The HAdV-D36 fiber knob domain (FK), which mediates the primary attachment of many HAdVs to host cells, has a significantly elongated DG loop that alters known binding interfaces for established adenovirus receptors such as the coxsackie- and adenovirus receptor (CAR) and CD46. Our data suggest that HAdV-D36 attaches to host cells using a versatile receptor pool comprising sialic acid-containing glycans and CAR. Sialic acids are recognized at the same binding site used by other HAdVs of species D such as HAdV-D37. Using glycan microarrays, we demonstrate that HAdV-D36 displays a binding preference for glycans containing a rare sialic acid variant, 4-O,5-N-diacetylneuraminic acid, over the more common 5-N-acetylneuraminic acid.

We employed glycan array screening with a library of about 500 glycans to identify SA-containing glycans that support efficient binding of the HAdV-D36 FK. Notably, HAdV-D36 FK demonstrated selective binding exclusively to 4-O-Ac-3’SL, contrasting with the preference of HAdV-D37 FK for 3’SL. Glycan probes containing a 3’SL motif capped with the unmodified Neu5Ac showed little or no binding. We solved the crystal structure of the HAdV-D36 fiber knob in complex with 4-O-Ac-3’SL isolated from echidna milk, and we observed that the lactose component is not ordered in two of the three complexed glycans and does not seem to contribute to the binding. The only detectable contact mediated by the glycan stem is formed between the poorly ordered O6 atom of the galactose moiety and a backbone carbonyl function. The lactose stem is generally poorly ordered and only partially visible in one of three cases.

>MSKRLRVEDDFNPVYPYGYARNQNIPFLTPPFVSSDGFQNFPPGVLSLKLADPIAIANGNVSLKVGGGLTVEQQSGKLSVDTKAPLQVANDNKLELSYDDPFKVENNKLGIKAGHGLAVVTKENTSLPSLVGTLVVLTGKGIGTGSSAHGGTIDVRLGEGGGLSFDEKGDLVAWDKKNDTRTLWTTPDPSPNCKVETARDSKLTLALTKCGSQILATVSLLVVTGKYAIISDTVNPKQFSIKLLFNDKGVLLSDSNLDGTYWNYRSNNNNIGTPYKEAVGFMPSTTAYPKPTNNTSTDPDKKVSQGKNKIVSNIYLGGEVYQPGFIVVKFNQETDANCAYSITFDFGWGKVYKDPIPYDTSSFTFSYIAQE[3x]> MNIRRKNRLWIACAVLAGLALTIGLVLYALRSNIDLFYTPGEILYGKRET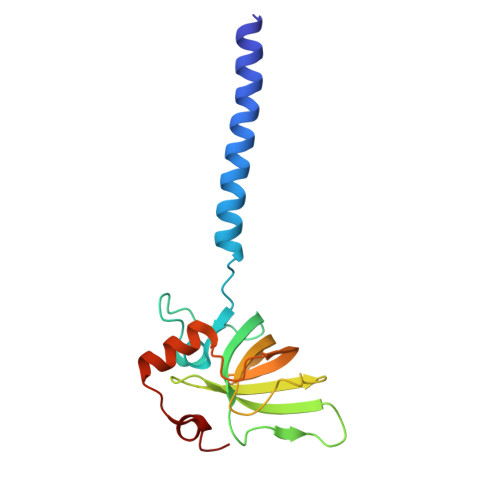QQMPEVGQRLRVGGMVMPGSVQRDPNSLKVTFTIYDAEGSVDVSYEGILPDLFREGQGVVVQGELEKGNHILAKEVLAKHDENYTPPEVEKAMEANHRRPASVYKDPAS> WCYEIQTEDPRSSCLGPEKWPGACKENQQSPINIVTARTKVNPRLTPFILVGYDQKQQWPIKNNQHTVEMTLGGGACIIGGDLPARYEAVQL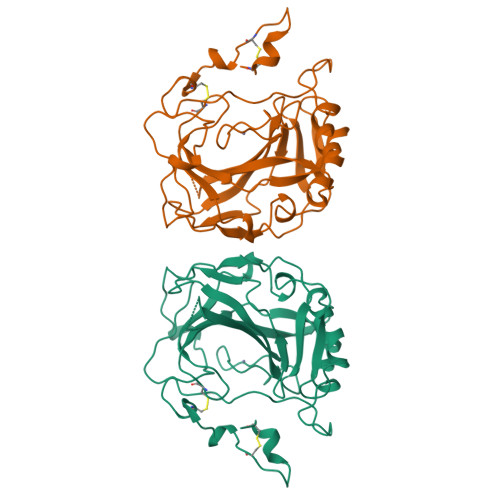HLHWSNGNDNGSEHSIDGRHFAMEMHIVHKKLTSSKEDSKDKFAVLAFMIEVGDKVNKGFQPLVEALPSISKPHSTSTVRESSLQDMLPPSTKMYTYFRYNGSLTTPNCDETVIWTVYKQPIKIHKNQFLEFSKNLYYDEDQKLNMKDNVRPLQPLGKRQVFKSHA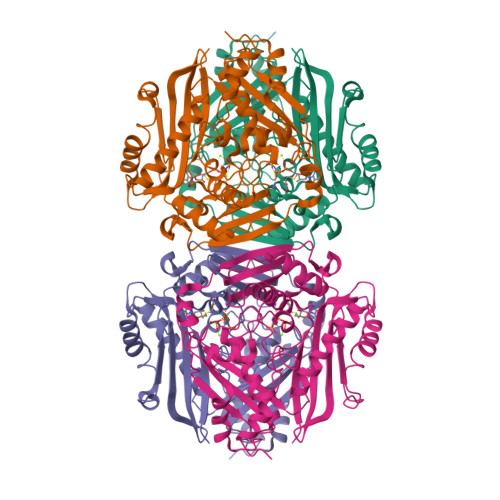>[4x]AKHLFTSESVSEGHPDKIADQISDAVLDAILEQDPKARVACETYVKTGMVLVGGEITTSAWVDIEEITRNTVREIGYVHSDMGFDANSCAVLSAIGKQSPDINQGVDRADPLEQGAGDQGLMFGYATNETDVLMPAPITYAHRLVQRQAEVRKNGTLPWLRPDAKSQVTFQYDDGKIVGIDAVVLSTQHSEEIDQKSLQEAVMEEIIKPILPAEWLTSATKFFINPTGRFVIGGPMGDCGLTGRKIIVDTYGGMARHGGGAFSGKDPSKVDRSAAYAARYVAKNIVAAGLADRCEIQVSYAIGVAEPTSIMVETFGTEKVPSEQLTLLVREFFDLRPYGLIQMLDLLHPIYKETAAYGHFGREHFPWEKTDKAQLLRDAAGLK>MDYKDDDDKMTSAQNESQALGDLAARQLANATKTVPQLSTITPRFLLHLLSWVPVEAGIYRVNRVVNPDRVAIHSEAGAGTEEPLPETYVDYETHPREYTLRSISTLLDVHTRVSDLYSSPHDQVTQQLRLTIETIKERQEYELVNNPEYGLLAQATPEQTIQTLAGAPTPDDLDALITKVWKTPAFFLTHPLGVAAFGRECTYRGVPPPTVSMYGAQFITWRGIPIVPSDKVPVEDGTTKFVLVRTGEERQGVVGLFQPGLVGEQAPGLSVRFTGINRSA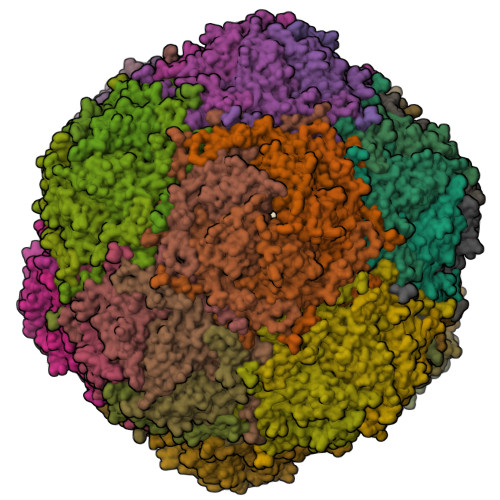IASYLVTLYTSLAVLTDDALAVLDGVAVDQFHEYQ[60x]> GASGSMNNMYLKAVIFSIADVVLPLTSNTQPQELKSRIDSELRKLFAFLSSKGIKVIFLTNKNRNVRTHDGIVTLDEYLKRKFPESIHFCRELDNNIPAKQTGKAIDFIMAALELKRNEMIYVGRSQEDLQAATNGNTLFINATWYEPVTEYGFQFSEPKEIARFIDVFCLREQLWGWQGHFNEDVHYYALAPFSTYVPEFTMYSANARDLAKLSVGSPDFWIRYLGASIYFSGLSEGASFITTYVGHNAEDPYKLANIMEHDLKGLAVSFKGKYLKDLFLRHTTAIKSQQARIAKQEVNITSQINTVNLNPAPIKNLIT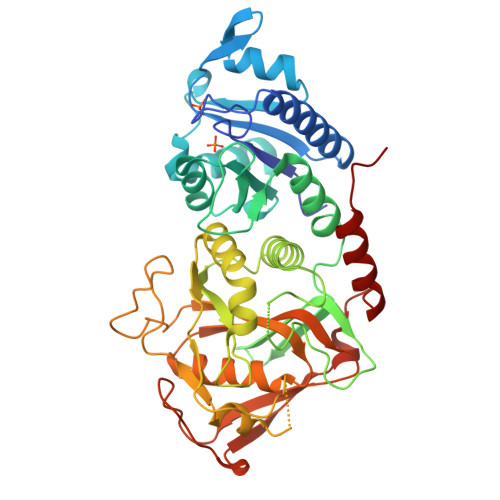GERYTNPPKLKGKKILVIDDFCTEGNAHETARMYLKAAGANVINISWLKTINRDVSICEPTRKIRPWEANTLDVDDINYVGTIGYAENVTHGSAPQVLSEKIQQYDNWDWPQ> SSALRDGYRQAGVSGRVRSYLDLLAGLSDFREHFDGSDGFSLDLVDMADGPGEVTVICCAGTAAISGPHEFTRLAGALRGIAPVRAVPQPGYEEGEPLPSSMAAVAAVQADAVIRTQGDKPFVVAGHSAGALMAYALATELLDRGHPPRGVVLIDVYPPG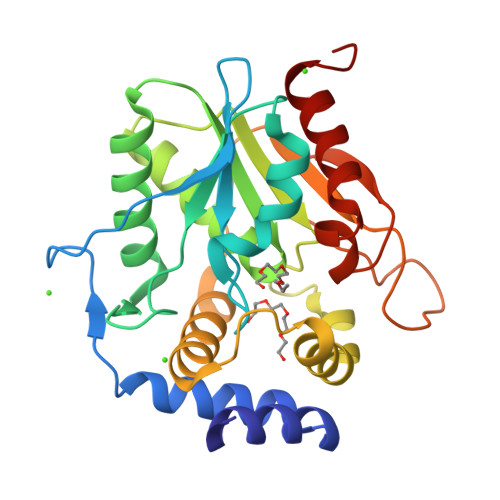HQDAMNAWLEELTATLFDRETVRMDDTRLTALGAYDRLTGQWRPRETGLPTLLVSAGEPMGPWPDDSWKPTWPFEHDTVAVPGDHFTMVQEHADAIARHIDAWLGGGNS2-(TRIMETHYLAMMONIUM)ETHYL THIOL | C5 H14 N 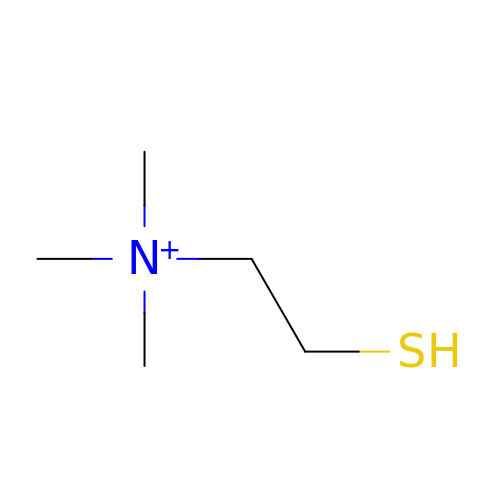S | VFUGTBZQGUVGEX-UHFFFAOYSA-O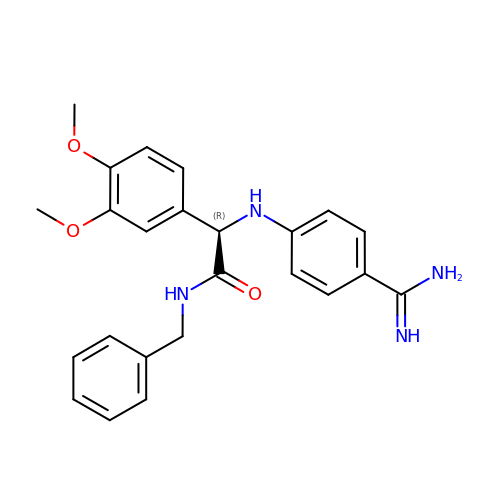(2R)-2-({4-[AMINO(IMINO)METHYL]PHENYL}AMINO)-N-BENZYL-2-(3,4-DIMETHOXYPHENYL)ACETAMIDE | C24 H26 N4 O3 | BMQMRSICTKGCCO-JOCHJYFZSA-N>GMESGFTSKDTYLSHFNPRDYLEKYYSFGSRHCAE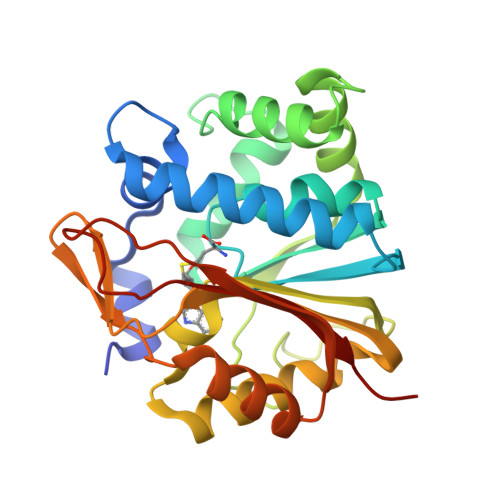NEILRHLLKNLFKIFCLGAVKGELLIDIGSGPTIYQLLSACESFTEIIVSDYTDQNLWELQKWLKKEPGAFDWSPVVTYVCDLEGNRMKGPEKEEKLRRAIKQVLKCDVTQSQPLGGVSLPPADCLLSTLCLDAACPDLPAYRTALRNLGSLLKPGGFLVMVDALKSSYYMIGEQKFSSLPLGWETVRDAVEEAGYTIEQFEVISQNYSSTTSNNEGLFSLVGRKPGRSE[4x]The transient receptor potential channel TRPM7 is a master regulator of the organismal balance of divalent cations that plays an essential role in embryonic development, immune responses, cell mobility, proliferation, and differentiation. TRPM7 represents a master regulator of the cellular balance of divalent cations and mediates uptake of Zn2+, Mg2+ and Ca2+, which is required for the normal prenatal development and healthy adulthood. The TRPM7 structure represents a tetramer assembled of four identical subunits, with the overall architecture reminiscent of other TRPM channels. Each TRPM7 subunit consists of an intracellular N-terminal domain (NTD, residues 1–789), transmembrane domain (TMD, 839–1146), and cytosolic C-terminal domain (CTD, 1157–1230).

To explore the agonist-induced TRPM7 activation structurally, we subjected the purified, nanodisc-reconstituted TRPM7 protein to single-particle cryo-EM in the presence of 1 mM NTB. Our data analysis revealed two distinct classes of particles. The second class of particles revealed by the processing of cryo-EM data collected from TRPM7 in the presence of NTB yielded a 2.44-Å resolution closed-state structure TRPM7NTB-Closed. This structure is very similar to TRPM7Closed, with the pore sterically sealed at the narrow constriction by the side chains of I1093 and N1097. Inspection of the cryo-EM map revealed four identical densities, one per subunit of TRPM7NTB-Closed tetramer, with the characteristic shape of NTB. Each of these densities unambiguously identified NTB binding sites located in the TMD region that faces the cytoplasmic leaflet of the membrane, at the interfaces between the S1–S4 and pore domains, distally from the NTB binding sites in TRPM7NTB-open. The sites in TRPM7NTB-Closed are contributed by the N-terminal part of S3, C-terminal part of S4, S4–S5 linker and TRP helix. Since the TRPM7NTB-Closed structure is nearly identical to the apo-state TRPM7Closed structure, the vanilloid-like site in TRPM7 does not serve as an activating binding site. Notably, a comparison of NTB molecules from TRPM7NTB-open and TRPM7NTB-closed structures shows that they are sterically identical and do not represent optical isomers (enantiomers).

>[4x]SQKSWIESTLTKRECVYIIPSSKDPHRCLPGCQICQQLVRCFCGRLVKQHACFTASLAMKYSDVKLGEHFNQAIEEWSVEKHTEQSPTDAYGVINFQGGSHSYRAKYVRLSYDTKPEIILQLLLKEWQMELPKLVISVHGGMQKFELHPRIKQLLGKGLIKAAVTTGAWILTGGVNTGVAKHVGDALKEHASRSSRKICTIGIAPWGVIENRNDLVGRDVVAPYQTLLNPLSKLNVLNNLHSHFILVDDGTVGKYGAEVRLRRELEKTINQQRIHARIGQGVPVVALIFEGGPNVILTVLEYLQESPPVPVVVCEGTGRAADLLAYIHKQTEEGGNLPDAAEPDIISTIKKTFNFGQSEAVHLFQTMMECMKKKELITVFHIGSEDHQDIDVAILTALLKGTNASAFDQLILTLAWDRVDIAKNHVFVYGQQWLVGSLEQAMLDALVMDRVSFVKLLIENGVSMHKFLTIPRLEELYNTKQGPTNPMLFHLIRDVKQGNLPPGYKITLIDIGLVIEYLMGGTYRCTYTRKRFRLIYNSLGGNNRRSGRNTSSSTPQLRKSHETFGNRADKKEKMRHNHFIKTAQPYRPKMDASMEEGKKKRTKDEIVDIDDPETKRFPYPLNELLIWACLMKRQVMARFLWQHGEESMAKALVACKIYRSMAYEAKQSDLVDDTSEELKQYSNDFGQLAVELLEQSFRQDETMAMKLLTYELKNWSNSTCLKLAVSSRLRPFVAHTCTQMLLSDMWMGRLNMRKNSWYKVILSILVPPAILMLEYKTKAEMSHIPQSQDAHQMTMEDSENNFHNITEEIPMEVFKEVKILDSSDGKNEMEIHIKSKKLPITRKFYAFYHAPIVKFWFNTLAYLGFLMLYTFVVLVKMEQLPSVQEWIVIAYIFTYAIEKVREVFMSEAGKISQKIKVWFSDYFNVSDTIAIISFFVGFGLRFGAKWNYINAYDNHVFVAGRLIYCLNIIFWYVRLLDFLAVNQQAGPYVMMIGKMVANMFYIVVIMALVLLSFGVPRKAILYPHEEPSWSLAKDIVFHPYWMIFGEVYAYEIDVCANDSTLPTICGPGTWLTPFLQAVYLFVQYIIMVNLLIAFFNNVYLQVKAISNIVWKYQRYHFIMAYHEKPVLPPPLIILSHIVSLFCCVCKRRKKDKTSDGPKLFLTEEDQKKLHDFEEQCVEMYFDEKDDKFNSGSEERIRVTFERVEQMSIQIKEVGDRVNYIKRSLQSLDSQIGHLQDLSALTVDTLKTLTAQKASEASKVHNEITRELSISKHLAQNLID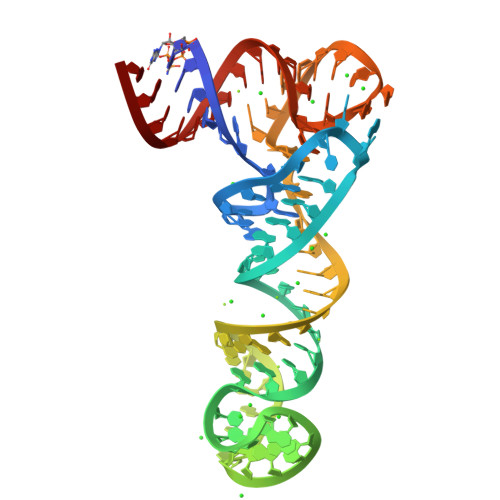> GCGGAAGUAGUUCAGUGGUAGAACACCUACUGGCCCGAAAGGGUGGAACCCCAGUAGGGGGUCGCGGGUUCGAGUCCCGUCUUCCGC>MELFDENYYAKAVANIIGEVKDPIMYKWFSPDQIEDVDLQMGYQKTVKWDAFLNANPTTIANEVNTISTIGFSSEVVRLNYLKLQYKFRHLKQTSEKFYTSDSYIGDINNNLLPFAQAYKLASSEIIKLINHFVLTGTVSIQKDGKNQKRLLPNMYGLLNMPEQIKEEVASGDKDKMDKIFEKIEAGLSKLELGDEFSTPMMVIVDPATSLKLVKPYAAAQGAASSCEKWEDVLIQTIKAINNREDVYIETSNLLKHKILIYPLNSELIKFKPSKYMLPTPNEQVDKDSTDVAHSYIDFVLGGLLATRKTILQVNIKQS[415x];>MSDITKIKQEFDKKVAEIQALMKNPQQDSGLLSNSIDFRDQNLIFSNSGGVCTSSKDKIENYPAKGYPYKRGVKLSFGDGTTELEVEAGGGDDLYGVCSDIDEFSGMATVIPITNNFTGYLTLKKDGQNGVNPGDKLNFNQHGELEKVTGAQKSVNAIALSKAHKLTEDLFIVLASVFGNRAIKG[280x];>[5x]MALKGNMQVENLEAVEDPQVDLGAQVSAAPRAKRQARQAEDVQGEDPYLESISELDDVLLKFKKYSKSMSSIENKVFSSSSGCFKSKNERVDAYSFACSSYTDKIEEYLYDPANSFPYKRGVKLVPKENSIYVEVGADTDMYGICVDVCEFSCTAYVLPITNNFEGYLVTRNPSIKIGEILDINNNGVIIKAGGGPPTAINIYALSDSFTINFAPEDGNQDQNRYPRQEYSINLIKVAIFGNRGLEKTVNPDGG;>MGDTTQLVKEYQEKRSKLEKFMKNPQHDASLLSNSNEFRDKNVEFFASGGTRTSKFDKLENHPFLGYPYKRGVKRVIQEAQDNQSHYEPHVEAGGGEDLYGICIDIDEFSKTATIVPITNNFEGYLVAKDSTVKVKDKLIFNKDGALEKVTGAPNKATINATALTDAKQISNEVYLVKVAVFGNKAMSRN[130x];>[826x]MTEKEEKEDLQAQDKEEQQIKADTKVISVQEFEEYMRFKEQANSKSKETSRDLSINERITKELAEVEERERIEKQLLLEAERINEIDTLAKAHLSNHFNKEVLLAKGYTLKDIMQAQRRELVRKFVPIEQIKAIAKVSDISHIDGEILEQLVSLAKVNIKLRKNASSSSSSVDSIKGNIAIKSEERASLLDSNFVPINFTEFVQAISNTYKQRRIQFYENLKRHKRTSIA;>MCDLRKTKLIDKISSLELYKYS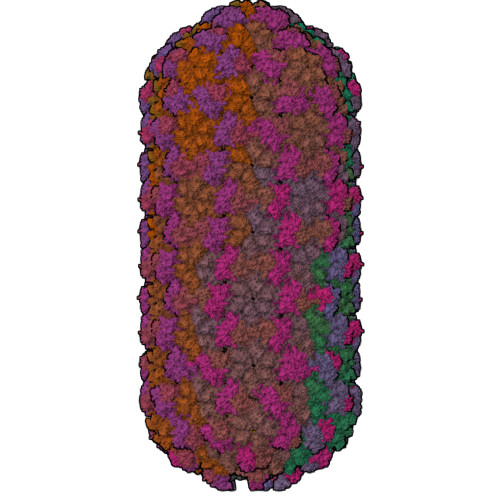IFFRNYIENVAEDCLKNGLILESAAHNVSEVELARLKVQLKNALLNCIISYRFHGIGYVLVKTKDTLIDLEQPVNIELPIGFEYLDYEYVRDLGVDFDHITYKVKSNNKNNSLDAVKIHKSRLIIYENFDYILKRYVPCYTESFLLDIYLFEKIYVEIERRIENHNFLFYKDESLVQLQDALSSATTSLSALTQSNNDRGSGILSSFLRKQNSNNHSKDISNLRNLNDSLSQELARLKSNLNNEGMFYTATPSASLEVIKYDLSYLKEALALIKAKIGADTKEPLTRSFNEQAKGLGNDGKGDRSNYYDFLKGVQEQVENSCNLKLTKYFGLDMKFNSLIMLSEEQKVERDIKLIELYSKYNQLIQSSSFNNEELAMLKEKLFSF[12x]> HHHHHHSDEALKMTMASVPAS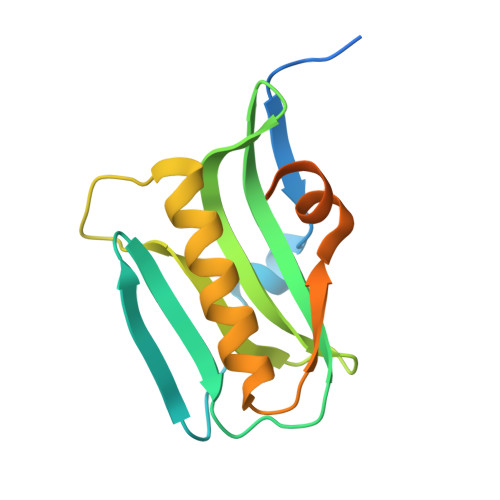RYLTDMTLEEMSRDWSMLIPKQKVAGPLCIRMDQAIMDKNIILKANFSVIFDRLETLILLRAFTEEGAIVGEISPLPSLPGHTAEDVKNAVGVLIGGLEWNDNTVRVSETLQRFAWRSSNENGRPPLTPKQKREMAGTIRSEV>[2x]SNAMSEEKSEEVQETRPTPRLNERILSSLSRRSVAAHPWHDLEIGPGAPNIFNCVVEITKGSKVKYELDKKTGMIKVDRILYSSVVYPHNYGFIPRTL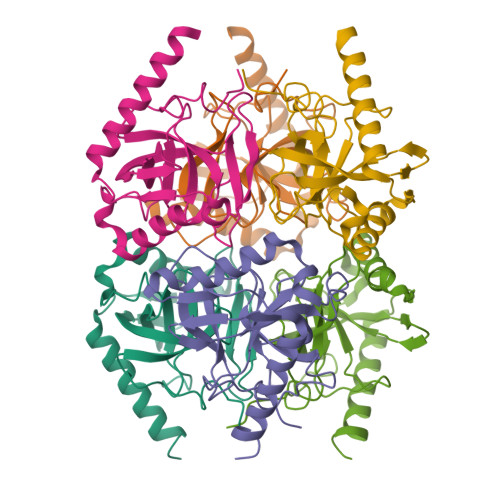CEDNDPLDVLVLMQEPVLPGCFLRARAIGLMPMIDQGEKDDKIIAVCADDPEYKHYTDFKELQPHRLMEIKRFFEDYKKNENKEVAVNEFLPPSTAVEAIQHSMDLYAEYILHTLR> MRYNQGCQLTAFFIGGNMKIVKHDGYNDIFNGGADGSPKPFFMSDASYHVGSFYNDNATAKRIVDVIPEEMVTAGFKISGVKDEKEFKSLWDSYKIDPSLVDALCWARLYGGAAIVAIINDNRMLTSPVKPGAKLEGVRVYDRFAITIEKRVTNARSPRYGEPEIYKVSPGDNIQPYLIHHTRIFIADGERVTPQMRKQNQGWGASVLNKSLIDAICDYDYCESLATQILRRKQQAVWKVKGLAEMCDDDDAQYAARLRLAQVDDNSGVGRAIGIDAETEEYDVLNSDISGVPEFLSSKMDRIVSLSGIHEIIIKNKNVGGVSASQNTALETFYKLVDRKREEDYRPLLEFLLPFIVDEQEWSIEFEPLSVPSKKEESEITKNNVESVTKAITEQIIDLEE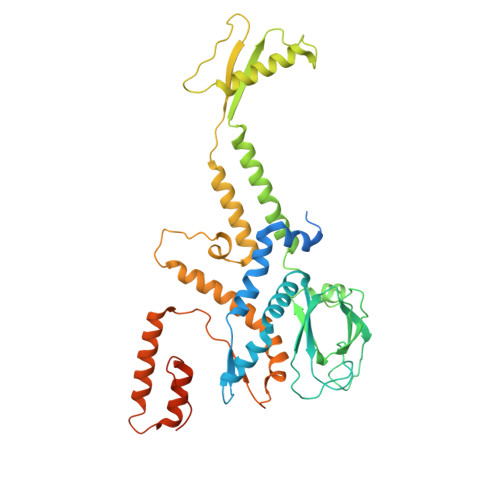ARDTLRSIAPEFKLKDGNNINIREPEEPTEPEPGLGEKLEDEN>[4x]MWSHPQFEKGSGSENLYFQGTMKVINDPIHGHIELHPLLVRIIDTPQFQRLRYIKQLGGGYYVFPGASHNRFEHSLGVGYLAGCLVHALGEKQPELQIS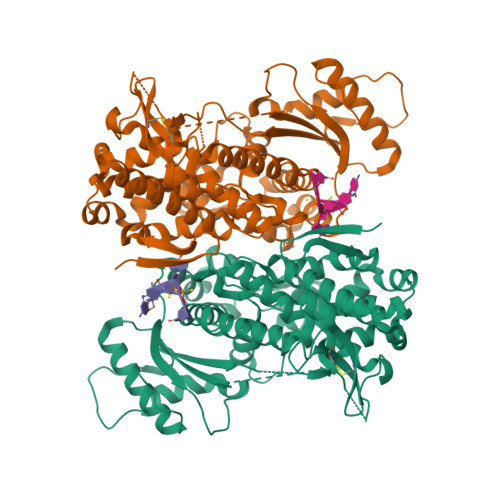ERDVLCVQIAGLCHDLGHGPFSHMFDGRFIPLARPEVKWTHEQGSVMMFEHLINSNGIKPVMEQYGLIPEEDICFIKEQIVGPLESPVEDSLWPYKGRPENKSFLYEIVSNKRNGIDVAKWDYFARDCHHLGIQNNFDYKRFIKFARVCEVDNELRICARDKEVGNLYDMFHTRNSLHRRAYQHKVGNIIDTMITDAFLKADDYIEITGAGGKKYRISTAIDDMEAYTKLTDNIFLEILYSTDPKLKDAREILKQIEYRNLFKYVGETQPTGQIKIKREDYESLPKEVASAKPKVLLDVKLKAEDFIVDVINMDYGMQEKNPIDHVSFYCKTAPNRAIRITKNQVSQLLPEKFAEQLIRVYCKKVDRKSLYAARQYFVQWCADRNFTKPQDGDVIAPLITPQKKEWNDSTSVQNPTRLREASKSRVQLFKDDPM>[3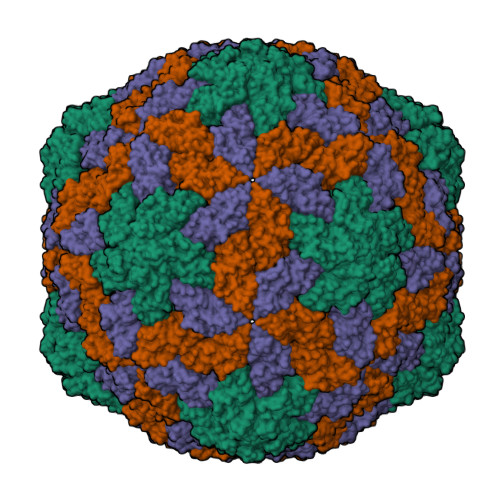x]MNSVGRRGPRRANQNGTRRRRRRTVRPVVVVQPNRAGPRRRNGRRKGRGGANFVFRPTGGTEVFVFSVDNLKANSSGAIKFGPSLSQCPALSDGILKSYHRYKITSIRVEFKSHASANTAGAIFIELDTACKQSALGSYINSFTISKTASKTFRSEAINGKEFQESTIDQFWMLYKANGTTTDTAGQFIITMSVSLMTAK3-METHYL-2-UREIDO-BUTYRIC 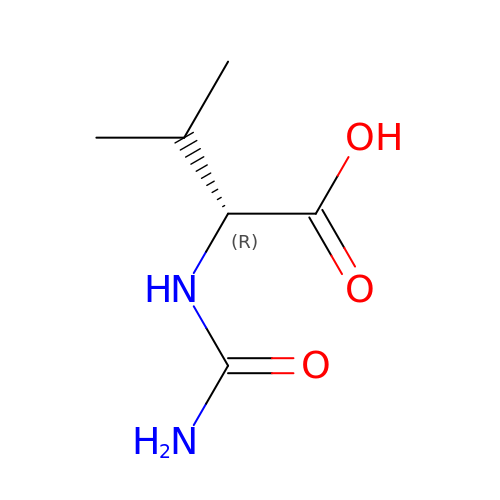ACID | C6 H12 N2 O3 | JDXMIYHOSFNZKO-SCSAIBSYSA-N>[2x]MEDPYIWMENLEDERVLKIIEEENKRFREFIGELSDKLFPE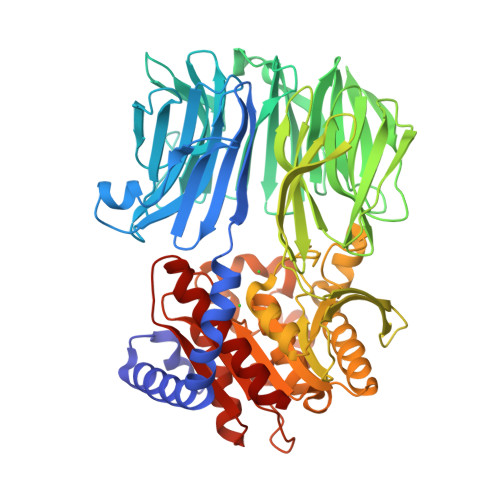VWEQFSQPTIGMARITKKGIIASYSEKDRVVIKWFNGDVIVDSKELEREVGDEVLLQGFTTDEEGEKLAYSFSIGGADEGITRIIDLKTGEVIEEIKPSIWNITFLKDGYYFTRFYRKEKTPDGVNPPAARMFWKDREGERMVFGEGLTSGYFMSIRKSSDGKFAIVTLTYGWNQGEVYIGPIDNPQEWKKVYSASVPVEAIDVVNGKLYILTKEGKGLGKIIAIKNGKIDEVIPEGEFPLEWAVIVRDKILAGRLVHASYKLEVYTLNGEKIKEITFDVPGSLYPLDKDEERVLLRYTSFTIPYRLYEFKDDLRLIEERKVEGEFRVEEDFATSKDGTKVHYFIVKGERDEKRAWVFGYGGFNIALTPMFFPQVIPFLKRGGTFIMANLRGGSEYGEEWHRAGMRENKQNVFDDFIAVLEKLKKEGYKVAAWGRCNGGLLVSATLTQRPDVMDSALIGYPVIDMLRFHKLYIGSVWIPEYGNPEDPKDREFLLKYSPYHNVDPKKKYPPTLIYTGLHDDRVHPAHALKFFMKLKEIGAPVYLRVETKSGHMGASPETRARELTDLLAFVLKTLS> GMIEKVYEFKRDAKTKVVEKLV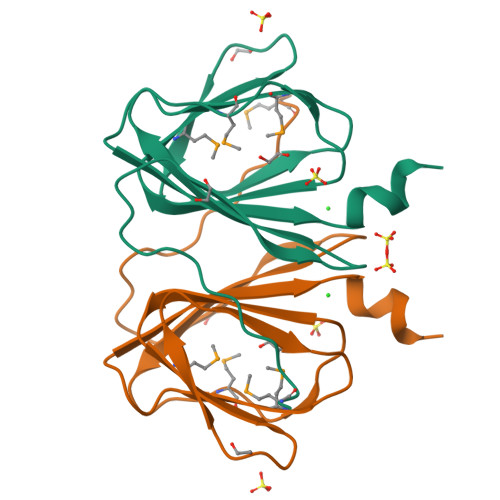NTEHVQINHIVLPRGEQMPKHYSNSYVHLIIIKGEMTLTLEDQEPHNYKEGNIVYVPFNVKMLIQNINSDILEFFVVKAPHPKKLNAPEDPIKCE> MQLREIRNCLLKCISECS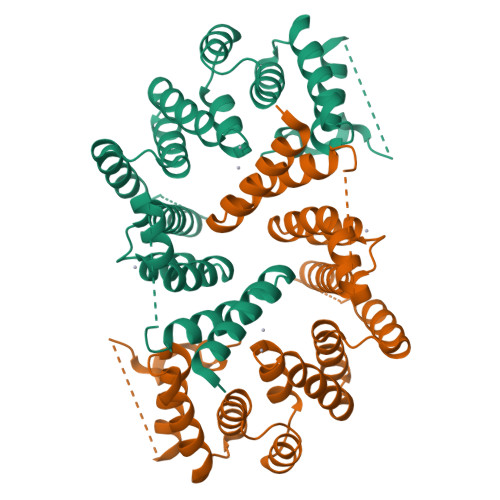ERGLVYAVRWAAEMLNGMNPIEMEHIPFSSTPTGEFDLDPDMANEKLLEVEEKNIYLLAKSYFDCKEFERAAYTLQNCKSSKSIFLRLYSKYLAGEKKSEEENETLLNTNLTLSSTNREFYYISEVLESLHYQGNKDPYLLYLSGVVYRKRKQDSKAIDFLKSCVLKAPFFWSAWLELSLSIDSLETLTTVVSQLPSTHIMTKIFYVYASHELHQVNSSAYEKLAEAEIIFPNSRYLKTQRALLTYDSRDFDEAESLFENILTNDPAENLYFQ Recent work has shown that the metal‐dependent protein phosphatase PPM1H counteracts LRRK2 by dephosphorylating Rabs. The crystal structure of PPM1H reveals a structurally conserved phosphatase fold that strikingly has evolved a 110‐residue flap domain adjacent to the active site. Cellular assays, crosslinking and 3‐D modelling suggest that the flap domain encodes the docking motif for phosphorylated Rabs. Therefore, PPM1H has acquired a Rab‐specific interaction domain within a conserved phosphatase fold.

In addition to the Mg2+ complexes, a structure of PPM1HWT (33‐514, loopDEL) with 3 Mn2+ ions was also determined at 2.2 Å resolution (MnPPM1HWT‐LD). However, all of the structures are identical with only minor differences arising from flexible loops and the presence or absence of the third metal ion at the active site. Phosphorylated Rab8a (pRab8a, GTP‐bound) from the recent structure of the pRab8a:RILPL2 complex (Waschbüsch et al, 2020) was docked onto PPM1H using Haddock software (Dominguez et al, 2003; van Zundert et al, 2016). The structure of MnPPM1HWT‐LD with 3 Mn2+ ions was used for docking with distance restraints applied between pThr72 of pRab8a and the metal ions of PPM1H. The structures of PPM1H with two Mg2+ ions failed to dock with pRab8a at the active site, presumably due to the density of negative charges in the absence of a third metal ion. The model reveals that the extended active site cleft involving the flap domain forms multiple interactions with pRab8A within the PPM1H active site. Overall, the crosslinking data and docking model are consistent with pRab8a recognition by the flap domain with phosphorylated Thr72 in the switch II motif oriented towards the active site for dephosphorylation. We also performed docking of the switch 2 α‐helical peptide from pRab8a with MnPPM1HWT‐LD. However, two of the top 10 solutions revealed a similar orientation of the phosphorylated switch 2 helix to the protein/protein dock. Overall, the complete 8/10 docking solutions of PPM1H/peptide and the top 5/6 docking solutions of PPM1H/protein suggest that the flap domain is very likely to contribute to substrate recognition (Fig EV2A and B).

>GSHMSDLPLRFPYGRPEFLGLSQDEVEASADHIARPILILKETRRLPWATGYAEVINAGKSTHNEDQASCEVLTVKKKAGAVTSTPNRNSSKRRSSLPNGEGLQLKENSESEGVSCHYWSLFDGHAGSGAAVVASRLLQHHITEQLQDIVDILKNSAVLGSGSTRFFTEKKIPHECLVIGALESAFKEMDLQIERERSSYNISGGCTALIVICLLGKLYVANAGDSRAIIIRNGEIIPMSSEFTPETERQRLQYLAFMQPHLLGNEFTHLEFPRRVQRKELGKKMLYRDFNMTGWAYKTIEDEDLKFPLIYGEGKKARVMATIGVTRGLGDHDLKVHDSNIYIKPFLSSAPEVRIYDLSKYDHGSDDVLILATDGLWDVLSNEEVAEAITQFLPNCDPDDPHRYTLAAQDLVMRARGVLKDRGWRISNDRLGSGDDISVYVIPLIHGNKLS[2x]>MSLCLPTIRKIAIIGAGPSGLVTAKALLAEKAFDQVTLFERRGSPGGVWNYTSTLSNKLPVPSTNPILTTEPIVGPAALPVYPSPLYRDLQTNTPIELM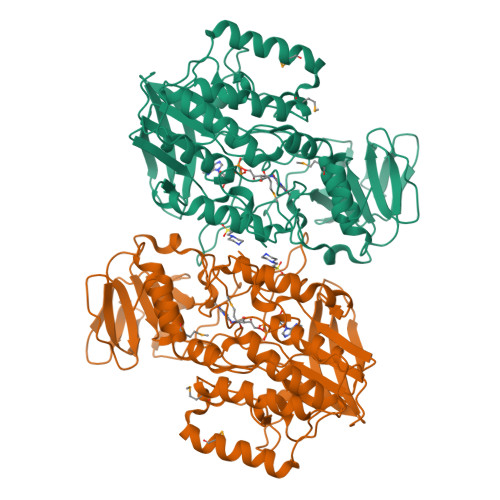GYCDQSFKPQTLQFPHRHTIQEYQRIYAQPLLPFIKLATDVLDIEKKDGSWVVTYKGTKAGSPISKDIFDAVSICNGHYEVPYIPNIKGLDEYAKAVPGSVLHSSLFREPELFVGESVLVVGGASSANDLVRHLTPVAKHPIYQSLLGGGDIQNESLQQVPEITKFDPTTREIYLKGGKVLSNIDRVIYCTGYLYSVPFPSLAKLKSPETKLIDDGSHVHNVYQHIFYIPDPTLAFVGLALHVVPFPTSQAQAAFLARVWSGRLKLPSKEEQLKWQDELMFSLSGANNMYHSLDYPKDATYINKLHDWCKQATPVLEEEFPSPYWGEKERSIRENMWSIRAKFFGIEPPKEGHHHHHH[2x]> MSRSKRDNNFYSVEIGDSTFTVLKRYQNLKPIGSGAQGIVCAAYDAILERNVAIKKLSRPFQNQTHAKRAYRELVLMKVVNHKNIIGLLNVFTPQKSLEEFQDVYIVMELMDANLSQVIQMELDHERMSYL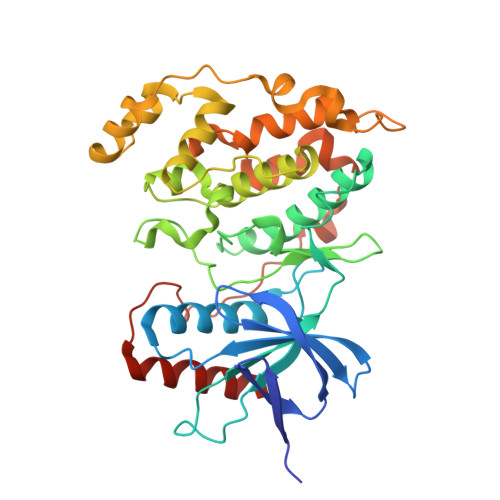LYQMLCGIKHLHSAGIIHRDLKPSNIVVKSDATLKILDFGLARTAGTSFMMTPYVVTRYYRAPEVILGMGYKENVDIWSVGCIMGEMIKGGVLFPGTDHIDQWNKVIEQLGTPSPEFMKKLQPTVRTYVENRPKYAGYSFEKLFPDVLFPADSEHNKLKASQARDLLSKMLVIDASKRISVDEALQHPYINVWYDPSEAEAPPPKIPDKQLDEREHTIEEWKELIYKEVMDLEHHHHHH Human cytochrome P450 (CYP) 2C9, a member of the CYP2C subfamily of CYP enzymes, is an important drug metabolizing enzyme and represents as much as ~20% of the total hepatic cytochrome P450 content. It is predominantly responsible for the biotransformation of many prescribed clinical drugs that include anti-coagulant (S)-warfarin, anti-hypertensive losartan, anti-convulsant phenytoin, anti-diabetics tolbutamide and glimepiride, as well as the commonly used analgesic ibuprofen. CYP2C9 is a highly polymorphic enzyme that includes over 60 classified genetic variants, with at least 20 reported to possess altered activity. The CYP2C9*8 genetic variant, predominantly found in individuals of African ancestry with an allele frequency of ~0.06, is a missense variant (449G>A) that is mostly associated with reduced enzyme activity towards various drug substrates.

The structure of CYP2C9*8 complexed with losartan clearly illustrates the amino acid change from R to H at position 150 (R150H) located on the surface of the protein. The sidechain of histidine at 150 is oriented towards the solvent and away from other secondary structural elements. On the other hand, the CYP2C9*8-losartan complex showed two molecules of losartan that include binding at the active site and the peripheral site, as observed in the WT complex, but lost one binding site in the access channel. The orientation of losartan in the active site and at the peripheral binding site is similar to that observed in the WT complex. The overall fold was conserved between the two structures with a root mean square deviation (RMSD) of 0.23 Å; however, the structures differed in the occupancy of losartan molecules. Furthermore, the structure of the *8 complex demonstrated the rotation of the H150 sidechain by about ~60° in an alternate conformation compared to the sidechain of R150 in the WT complex. The active site losartan has a biphenyl ring located near the heme, while the tetrazole and the imidazole rings were oriented near the helices away from the heme. Interestingly, the structural overlay of CYP2C9*2, *3, *8 and WT complexes of losartan revealed that the F476 sidechain in the *8 structure rotates ~30° towards the access channel compared to that observed in the WT structure. On the other hand, the average KD for losartan binding to CYP2C9*8 was 8.95 ± 0.97 µM, which was comparable to that yielded previously by the *2 variant (9.0 ± 0.5 µM). Importantly, the orientation of losartan in the active site of CYP2C9*8 is inconsistent with the demonstrated metabolism as the site of hydroxylation of losartan is located further away from the heme iron.

> MAKKTSGRGKLPPGPTPLPVIGNILQIGIKDISKSLTNLSKVYGPVFTLYFGLKPIVVLHGYEAVKEALIDLGEEFSGRGIFPLAERANRGFGIVFSNGKKWKEIRRFSLMTLRNFGMGKRSIEDRVQEEAHCLVEELRKTKASPCDPTFILGCAPCNVICSIIFHKRFDYKDQQFLNLMEKLNENIKILSSPWIQICNNFSPIIDYFPGTHNKLLKNVAFMKSYILEKVKEHQESMDMNNPQDFIDCFLMKMEKEKHNQPSEFTIESLENTAVDLFGAGTETTSTTLRYALLLLLKHPEVTAKVQEEIERVIGRNRSPCMQDRSHMPYTDAVVHEVQRYIDLLPTSLPHAVTCDIKFRNYLIPKGTTILISLTSVLHDNKEFPNPEMFDPHHFLDEGGNFKKSKYFMPFSAGKRICVGEALAGMELFLFLTSILQNFNLKSLVDPKNLDTTPVVNGFASVPPFYQLCFIPIHHHH>[2x]LEKRPRLVGGDIPCSGRVEVKHGDTW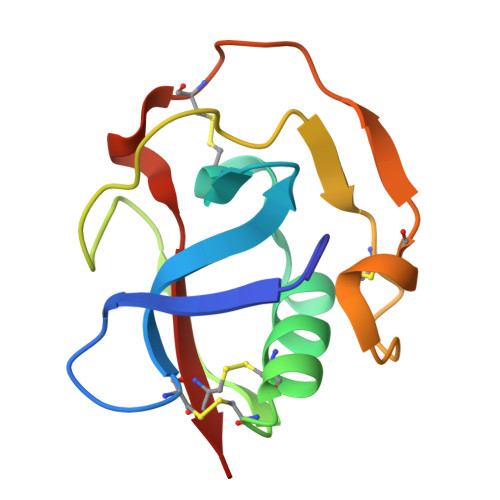GSVCDSDFSLEAASVLCRELQCGTVVSILGGAHFGEGNGQIWTEEFQCEGHESHLSLCPVAPRPEGTCSHSRDVGVVCSVD>MHHHHHHLVRPRGSHMTNSTDGRADGRLRVVVLGSTGSIGTQALQVIADNPDRFEVVGLAAGGAHLDTLLRQRAQTGVTNIAVADEHAAQRVGDIPYHGSDAATRLVEQTEADVVLNALVGALGLRPTLAALKTGARLALANKESLVAGGSLVLRAARPGQIVPVDSEHSALAQCLRGGTPDEVAKLVLTASGGPFRGWSAADLEHVTPEQAGAHPTWSMGPMNTLNSASLVNKGLEVIETHLLFGI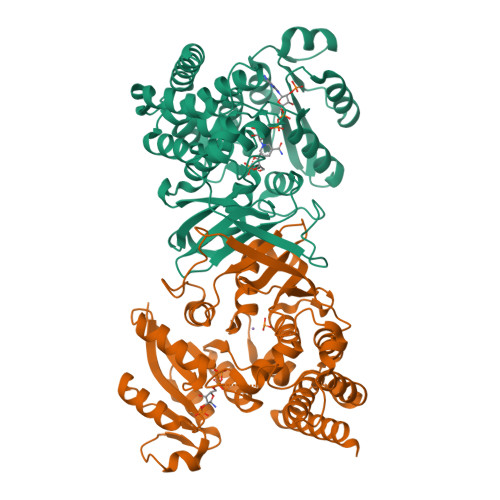PYDRIDVVVHPQSIIHSMVTFIDGSTIAQASPPDMKLPISLALGWPRRVSGAAAACDFHTASSWEFEPLDTDVFPAVELARQAGVAGGCMTAVYNAANEEAAAAFLAGRIGFPAIVGIIADVLHAADQWAVEPATVDDVLDAQRWARERAQRAVSGM[2x]N,N-BIS(3-AMINOPROPYL)-2-ANTHRAQUINONESULFONAMIDE | C20 H25 N3 O4 S | 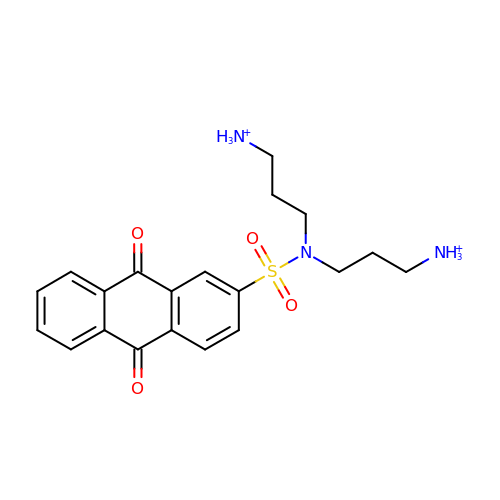HUHBNNVFLMYFIE-UHFFFAOYSA-P Among the five L,D-transpeptidase paralogs of M.tb, LdtMt2 plays an important role since an M.tb strain lacking the gene encoding this enzyme exhibits attenuation in virulence and exhibits enhanced susceptibility to β-lactam antibiotics. The L,D-transpeptidase class in M.tb is comprised of at least four substructural domains including two immunoglobulin-like domains (IgD1 and IgD2), a YkuD domain, and a C-terminal subdomain (CTSD). The YkuD domain has a highly conserved motif HXX14-17[S/T]HGChN containing three residues analogous to the catalytic triad of cysteine proteases: a cysteine, a histidine and a third residue (Cysteine 354, Histidine 336, and Serine 337 in LdtMt2) to catalyse the transpeptidation reaction. Based on our structural, biophysical, and biochemical data, we identify a new PG disaccharide moiety-binding pocket (named as S-pocket) at a distance of 21 Å from the catalytic site in LdtMt2.

The crystal structure of LdtMt2 was solved at 1.57 Å resolution. This high-resolution crystal structure is an improvement of our previous efforts that enabled us to identify an electron density in a pocket between the IgD2-YkuD domains, and a glucose molecule could be modelled into the electron density at 1.0 sigma. The sugar molecule is ensconced at the IgD2-YkuD domain interface in a pocket, which we referred to as the S-pocket, making several electrostatic interactions with residues R209, E207, E168, R371, Y330, and A171. Three residues M157, A171, and L391 stabilize the sugar through hydrophobic interactions. Superposition of the structures of the LdtMt2–sugar complex with the LdtBS–PG complex suggests that longer nascent PG chains thread across the S-pocket in between the IgD1-YkuD domains of LdtMt2. Based on the structural details of PG binding in LdtBS and LdtMt2, a PG chain was computationally placed over a positively charged surface across the IgD2-YkuD domain interface encompassing the S-pocket. This computational modelling of a longer PG chain spatially aligns one of its tetrapeptide stem across an inner cavity of the catalytic site in YkuD domain in LdtMt2, similar to reports of carbapenem and a PG-moiety binding in the same position. Based on our crystal structure and modelling study, we propose that the S-pocket anchors the disaccharide moiety of one of the nascent PG chains prior to transpeptidation of tetrapeptide stems in the catalytic site.

>[2x]GHMAPIKVIADKGTPFADLLVPKLTASVTDGAVGVTVDAPVSVTAADGVLAAVTMVNDNGRPVAGRLSPDGLRWSTTEQLGYNRRYTLNATALGLGGAATRQLTFQTSSPAHLTMPYVMPGDGEVVGVGEPVAIRFDENIADRGAAEKAIKITTNPPVEGAFYWLNNREVRWRPEHFWKPGTAVDVAVNTYGVDLGEGMFGEDNVQTHFTIGDEVIATADDNTKILTVRVNGEVVKSMPTSMGKDSTPTANGIYIVGSRYKHIIMDSSTYGVPVNSPNGYRTDVDWATQISYSGVFVHSAPWSVGAQGHTNTSHGCLNVSPSNAQWFYDHVKRGDIVEVVNTVGGTLPGIDGLGDWNIPWDQWRAGNAKA>GSHMSELEKAMVALIDVFHQYSGREGDKHKLKKSELKELINNELSHFLEEIKEQEVVDKVMETLDNDGDGECD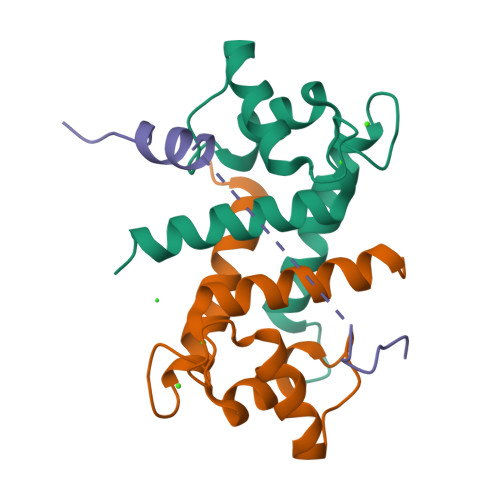FQEFMAFVAMVTTACHEFFEHE[2x];> GSGAMAATYSALNSSKPTPQLKPIESSILAQRRVRKLPSTTL>MSAKKIVLKSSDGESFEVEEAVALESQTIAHMVEDDCVDNGVPLPNVTSKILAKVIEYCKRHVEAAASKAEAVEGAATSDDDLKAWDADFMKIDQATLFELILAANYLNIKNLLDLTCQTVADMIKGKTPEEIRTTFNIKNDFTPEEEEEVRRENQWAFE[2x];>[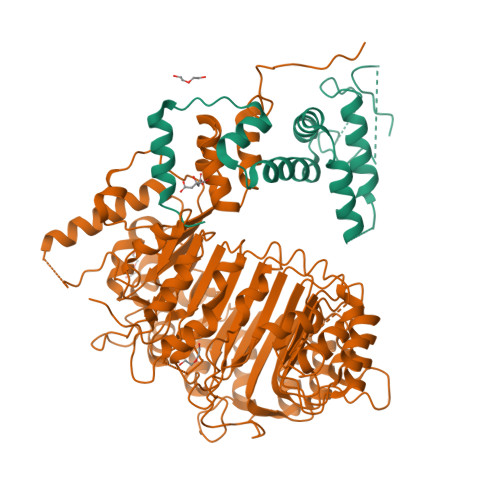2x]MAEEEEVEEGRSSSSAILDLPEPLLLHILSFLTDVRSRHRAALACGRMRAAERATRSELSLRGDPRSPGFLFLSHAFRFPALEHLDLSLVSPWGHPLLSSVPPCGGGGGGAPSASSSSGMNVYHPEAISEQNAFIAARLAGCFPAVTSLAVYCRDPTTLANLTPHWQASLRRVKLVRWHQRPPTLPDGADLEPLLETCAALRELDLSEFYCWTEDVVRALTTHPSATAALTHLDLGLAAATDGFKSSELGPIAASCPNLRKLVAPCLFNPRFSDCVGDDALLSLATSCPRLTVLRLSEPFEAAANIQREEAAITVAGLVAFFAALPALEDFTMDLQHNVLEAAPAMEALARRCPRIKFLTLGSFQGLCKASWLHLDGVAVCGGLESLYMKNCQDLTDASLAAIGRGCRRLAKFGIHGCDLVTSAGIRRLAFTLRPTLKEVTVLHCRLLHTAECLTALSPIRDRIESLEINCVWNTTENLYFQSLGSWEMLRSLSLWFSAGQLLSPLISAGLDSCPVLEEISIKVEGDCRTCPRPAPRTIFGLSDLAGFPVLAKMKLDLSEAVGYALTAPTGQMDLSLWERFYLHGIESLQTLYELDYWPPQDKDVHHRSLTLPAVGLIQRCVGLRKLFIHGTTHEHFMTFFLSIPNLRDMQLREDYYPAPENDLMFTEMRAESWLRFEVQLNSRQIDK> MGAQVTRQQTGTHENANIATNGSHITYNQINFYKDSYAASASKQDFSQDPSKFTEPVVEGLKAGAPVLKSPSAEACGYSDRVLQLKLGNSAIVTQEAANYCCAYGEWPNYLPDHEAVAIDKPTQPETATDRFYTLKSVKWETESTGWWWKLP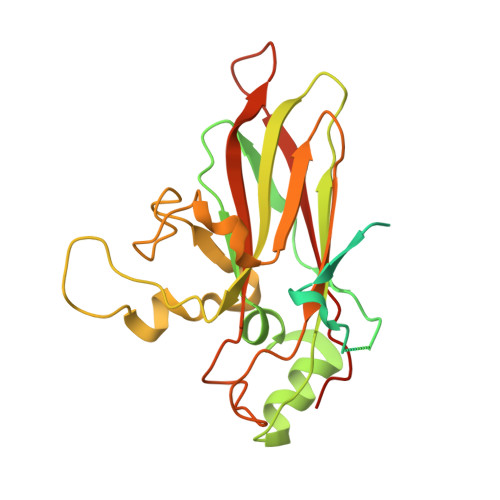DALNNIGMFGQNVQHHYLYRSGFLIHVQCNATKFHQGALLVVAIPEHQRGAHNTTTSPGFDDIMKGEEGGTFNHPYVLDDGTSLACATIFPHQWINLRTNNSATIVLPWMNAAPMDFPLRHNQWTLAIIPVVPLGTRTVSSMVPITVSIAPMCCEFNGLRHAITQ[1-oxidanyl-2-[3-[3-[[3-[[3-[3-(2-oxidanyl-2,2-diphosphono-ethyl)phenyl]phenyl]sulfamoyl]phenyl]sulfonylamino]phenyl]phenyl]-1-phosphono-ethyl]phosphonic acid 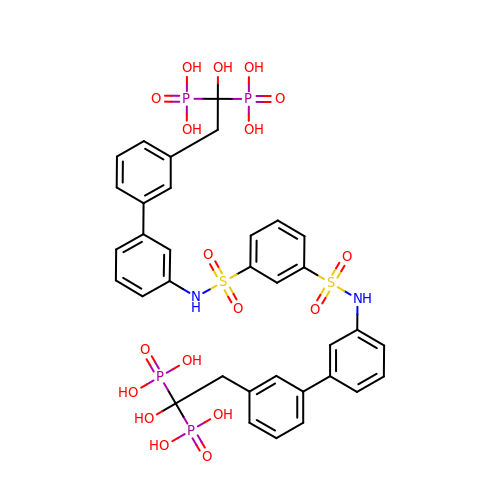| C34 H36 N2 O18 P4 S2 | UKSQFLAKPJZXNT-UHFFFAOYSA-N[(2~{S},5~{R})-1-[(2~{R},3~{S},4~{R},5~{R})-5-(6-aminopurin-9-yl)-3,4-bis(oxidanyl)oxolan-2-yl]-5-azaniumyl-6-oxidanyl-6-oxidanylidene-hexan-2-yl]-(3-oxidanylpropyl)azanium | C18 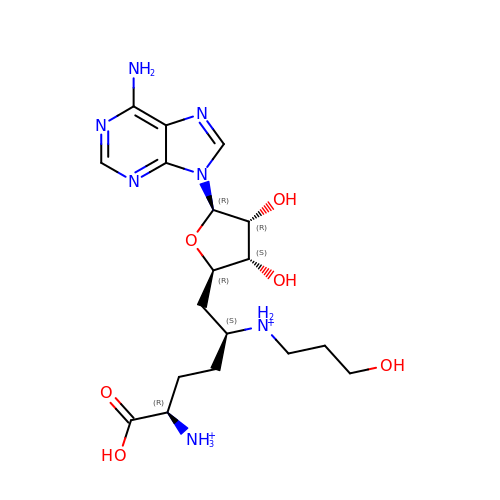H31 N7 O6 | UXRCPBKKSMEZKD-BRZDOZMNSA-P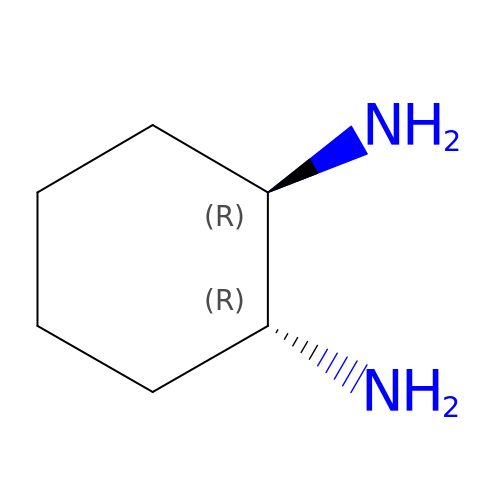1R,2R-DIAMINOCYCLOHEXANE | C6 H14 N2 | SSJXIUAHEKJCMH-PHDIDXHHSA-N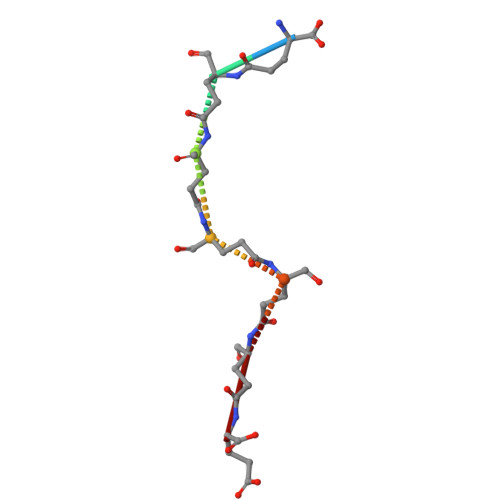> EEEEEEE>[3x]GQDSTSDLIPAPPLSKVPLQQNFQDNQFQGKWYVVGLAGNAILREDKDPQKMYATIYELKEDKSYNVTSVLFRKKKCDYWIRTFVPGSQPGEFTLGNIKS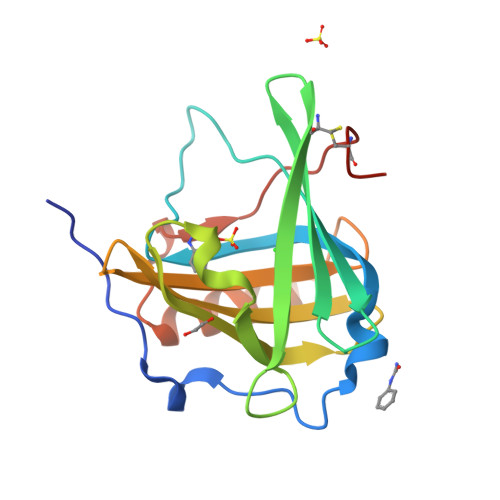YPGLTSYLVRVVSTNYNQHAMVFFKKVSQNREYFKITLYGRTKELTSELKENFIRFSKSLGLPENHIVFPVPIDQCIDGIVTD>MEIIPSESHPHIQLLKSNRELLVTHIRNTQCLVDNLLKNDYFSAEDAEIVCACPTQPDKVRKILDLVQSKGEEVSEFFLYLLQQL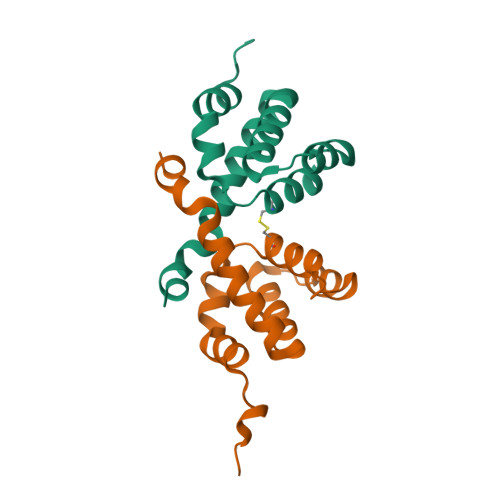ADAYVDLRPWLLE[2x]>[2x]ELHHHHHHMTDKTLQQIDKLICSWLKQIDNVIPQLI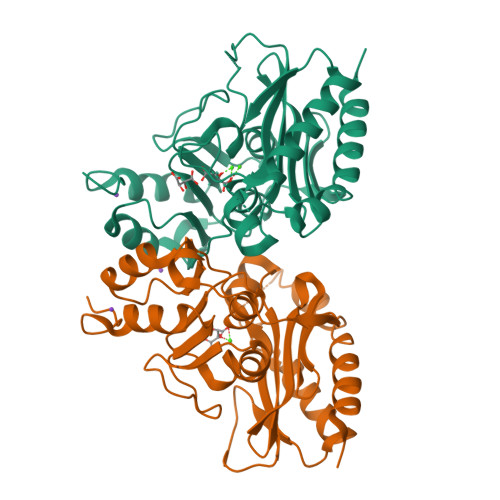MEMTTETKRHRFDLVTNVDKQIQQQFQQFLATYFPEHQLLAEEKSNAMITNEINHLWIMDPIDGTANLVKQQEDYCIILAYFYEGKPMLSYVYDYPHKKLYKAIRGEGAFCNGIKMEEPPSLKLEDAIISFNAQVMNLDTVQDLFDASFSYRLVGACGLDSMRVAKGQFGAHINTNPKPWDIAAQFLFAELLNLKMTTLDGKAIDHLKGAPFIISNKACHETVLKILNANGGYQKYR Cellulase 9I (Cel9I), is a non-cellulosomal family 9 processive endoglucanase from Clostridium thermocellum, which degrades crystalline cellulose (Avicel and filter paper) as well as phosphoric acid-swollen cellulose (PASC) and carboxymethyl cellulose (CMC). This enzyme consists of a catalytic GH9 module at its N terminus, followed by two family 3 carbohydrate-binding modules (CBMs): CBM3c and CBM3b. The C-terminal CBM3b module, as a classic CBM3, is responsible for targeting the Cel9I enzyme to the planar surface of the crystalline cellulose substrate (Gilad et al., 2003; Su, Mackie & Cann, 2012; Tormo et al., 1996). Thus, Gilad et al., showed in 2003 that the endoglucanase activity of Cel9I is dependent upon the presence of the CBM3c module and suggested that the fused CBM3c serves an important accessory role for the catalytic domain by altering its character to facilitate processive cleavage of recalcitrant cellulose substrates.

The effect of the re-association of the CBM3c with linker (CBM3cL) and the CBM3c without linker (CBM3cNL) on the enzymatic activity of GH9 has been studied by the crystallization and structure determination of the reassembled GH9-CBM3cL complex at a resolution of 1.68 Å. Surprisingly, the combined modules crystallized and formed a structure similar to those of the known GH9 cellulases. The catalytic module of the Cel9I enzyme consists of residues 1–446, comprising 15 α-helices, whereby the twelve longest ones form the (α/α)6-barrel. One calcium ion is found near the catalytic cleft of the GH9 module of Cel9I and is coordinated by a Ser 210 (OG) 2.6 Å, Gly 211 (O) 2.4 Å, Asp 261 (O) 2.4 Å, Asp 214 bifurcated (OD1, OD2) 2.5 Å, and Glu 215 bifurcated (OD1, OD2) 2.5 Å. The CBM3c module consists of 150 amino acids arranged in an eight β-stranded sandwich motif homologous to other known family 3 CBM structures (Gilbert, Knox & Boraston, 2013; Mandelman et al., 2003; Petkun et al., 2010b; Sakon et al., 1997; Shimon et al., 2000; Tormo et al., 1996; Yaniv et al., 2014; Yaniv et al., 2012b; Yaniv et al., 2011). One calcium ion was found in the upper β-sheet of the CBM3c molecule and is coordinated by a water molecule and five residues from the upper β-sheet: Asn 500 (O), Glu 503 bifurcated (OE1, OE2), Asn 573 (O), Asn 576 (OD1), Asp 577 (OD1). The in vitro reassembled GH9-CBM3cL complex has a large intermodular interface, the contact area of which is 1,108.3 Å2, corresponding to 12.3% of the total surface-exposed area of the CBM3c module and 6.2% of the exposed GH9 module. Conserved residues of the linker (which spans from Gly447 to Asp462) make numerous contacts with conserved residues of the GH9 module, emphasizing the importance of the linker in this interaction.

> MENKNGGYLPEEEIPDQPPATGAFNYGEALQKAIFFYECQRSGKLDSSTLRLNWRGDSGLDDGKDAGIDLTGGWYDAGDHVKFNLPMSYSAAMLGWAVYEYEDAFKQSGQYNHILNNIKWACDYFIKCHPEKDVYYYQVGDGHADHAWWGPAEVMPMERPSYKVDRSSPGSTVVAETSAALAIASIIFKKVDGEYSKECLKHAKELFEFADTTKSDDGYTAANGFYNSWSGFYDELSWAAVWLYLATNDSSYLDKAESYSDKWGYEPQTNIPKYKWAQCWDDVTYGTYLLLARIKNDNGKYKEAIERHLDWWTTGYNGERITYTPKGLAWLDQWGSLRYATTTAFLACVYSDWENGDKEKAKTYLEFARSQADYALGSTGRSFVVGFGENPPKRPHHRTAHGSWADSQMEPPEHRHVLYGALVGGPDSTDNYTDDISNYTCNEVACDYNAGFVGLLAKMYKLYGEL;> MGSPDPKFNGIEEVPEDEIFVEAGVNASGNNFIEIKAIVNNKSGWPARVCENLSFRYFINIEEIVNAGKSASDLQVSSSYNQGAKLSDVKHYKDNIYYVEVDLSGTKIYPGGQSAYKKEVQFRISAPEGTVFNPENDYSYQGLSAGTVVKSEYIPVYDAGVLVFGREPLEHHHHHH>GMAEDMAADEVTAPPRKVLIISAGASHSVALLSGDIVCSWGRGEDGQLGHGDAEDRPSPTQLSALDGHQIVSVTCGADHTVAYSQSGMEVYSWGWGDFGRLGHGNSSDLFTPLPIKALHGIRIKQIACGDSHCLAVTMEGEVQSWGRNQNGQLGLGDTEDSLVPQKIQAFEGIRIKMVAAGAEHTAAVTEDGDLYGWGWGRYGNLGLGDRTDRLVPERVTSTGGEKMSMVACGWRHTISVSYSGALYTYGWSKYGQLGHGDLEDHLIPHKLEALSN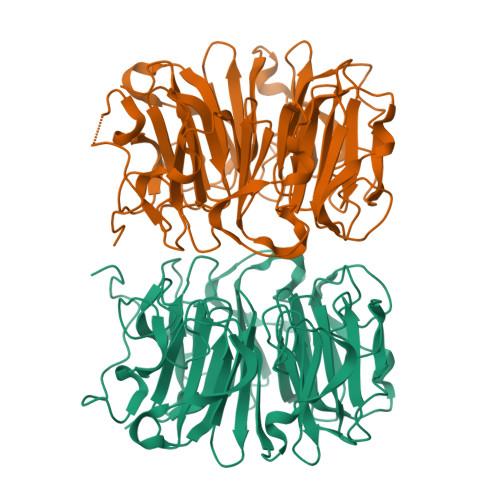SFISQISGGWRHTMALTSDGKLYGWGWNKFGQVGVGNNLDQCSPVQVRFPDDQKVVQVSCGWRHTLAVTERNNVFAWGRGTNGQLGIGESVDRNFPKIIEALSVDGASGQHIESSNIDPSSGKSWVSPAE[2x]> MHSSHHHHHHSSENLYFQGGGHMIHKLADVQSKNIGSGTRIWQFCVVLPSAIIGENCNICSHCFIEN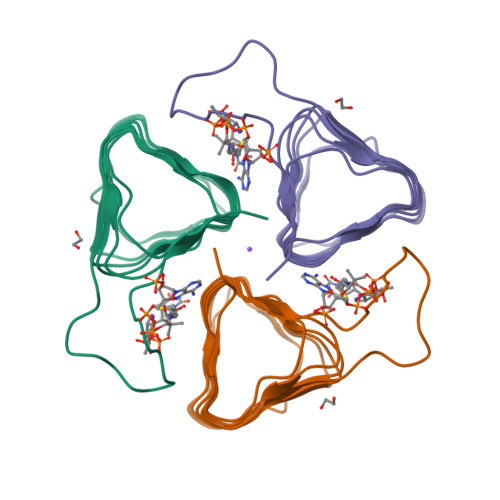DVKIGNNVTIKCGVQIWDGIEIEDDVFIGPNVTFTNDKYPRSKQYPKEFSKTIIKKGASIGANATILPGITIGENAMIGAGAIVTKDVLPHVTYYSKI> MPALTKSQTDRLEVLLNPKDEISLNSGKPFRELESELLSRRKKDLQQIYAEERENYLGKLEREITRFFVDRGFLEIKSPILIPLEYIERMGIDNDTELSKQIFRVDKNFCLRPMLAPNLANYLRKLDRALPDPIKIFEIGPCYRKESDGKEHLEEFTMLAFAQMGSGCTRENLESIITDFLNHLGIDFKIVGDSCMVFGDTLDVMHGDLELSSAVVGPIPLDREWGIDKPWIGAGFGLERLLK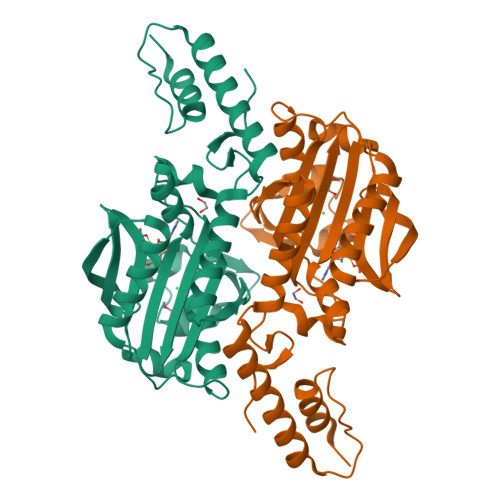VKHDFKNIKRAARSESYYNGISTNLHHHHHH>[10x]XGEIAQTLKEQA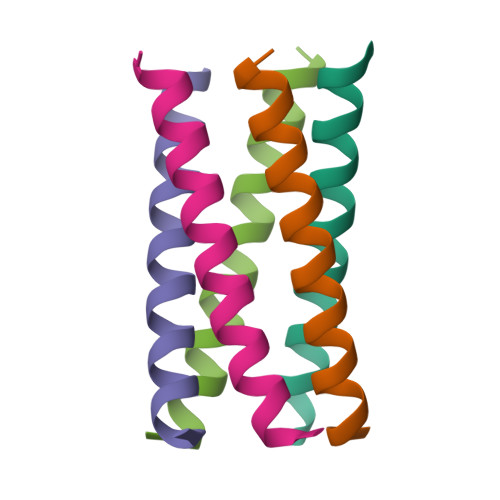KTLKEIAWTLKEIAQTLKGX>MIVTVINQKGGVGKTTTSVNLSYYLSKEKKTGLLDLDPEGGATISYGMKRELKELPLGEKSVNIFNVEVFPAHIGLLKLELNGDVEEISNKIKEIGKQFDFLVIDTPPNLGTLAISAMLVADRIVSPVTPQPLALEAIKNLDSRLKSIGKNAYSFTNFSKKVVKLDNLSSVKFTEITIPPSRLFIEAS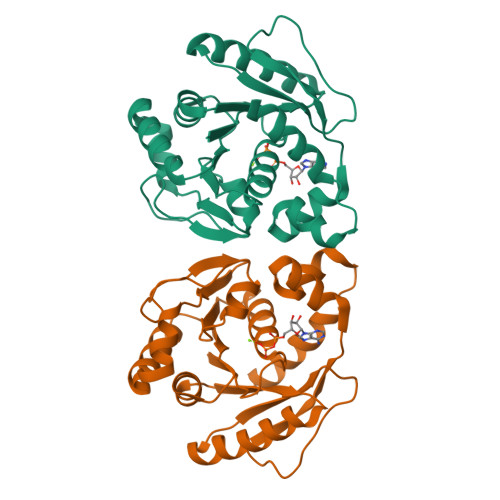RLGVPALRYEEVRIKKPKLANYYQQLAKVISE[4x]> GSMGKSHKCDFTKEKYLLSGEKEVSCEIDANPADDITFICPNKIDSLCFHTVNIAKNINQNKATMSIQDLLYGSVVYGNTLFISPYVRTNTPFYCFCNLDTVTIQKFLKINRFLKDDDELSEADVMKHLKGGNVAEAQADEYLNKALNRFKKMKDLSKFFNDQADNTAKLNLPKSLNIPNDILNYDVYNSANNRNDIVVKDEVTNKQIISKRGIMSVFVRS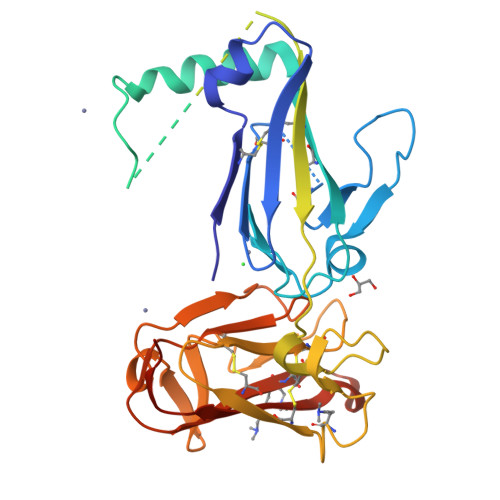NNNVIKGCDFGNNNKNYFSHPISVAGKVNNKVCKIQGKPGELVGFKCAFEENGKVEPPNCFDQVLHKNKVTDLKTLIPGYASYTNKHSSKYPYYLKIPHFVNEQYTIQCKCKSNNAQNEYTFELDIQPGESEVVLNSFKTSAAA> MLPPDILENGEFETIYFQTNPTYIKSPIHIPKSTIGKPDTVKIRHFFALLHQDLVVLGLEVFVYLQIYSDFVEKYVYVSKCDTVGLEKSTIKWGKVIGPVLQYIINYNGYKIKMKNLDEKSKDLSDPSTLVRLQRLRDKLPDIYPNLPYYNDIPPKEECIEYRTLPKTQNLRLCVFTKPAKEYLFPNSAKNPYKNLWNGQSLLRWWISIIDSITKGWNNHKLMIPGADKYATRKFIEKYSDWSEGHIFKKDGLAVQAIPLFPDDPKGRFLELVIVECRYGKMTVSRFYQELAYRQEFLLGDCVSLIGCCKENLEVTYHDDLVSTVTISEYKEFMNLLKL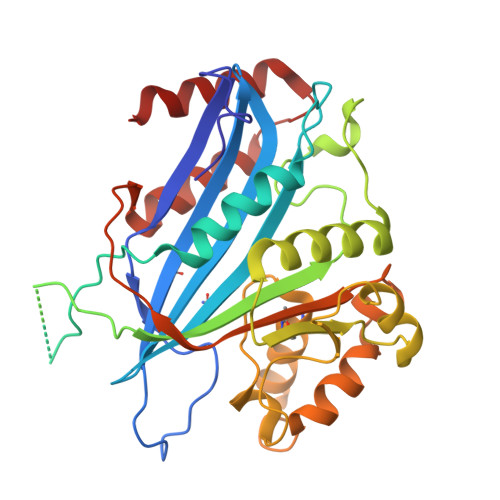VDFSDRVEVSNFVSNYRKSK>[2x]MKGQETRGFQSEVKQLLHLMIHSLYSNKEIFLRELISNASDAADKLRFRALSNPDLYEGDGELRVRVSFDKDKRTLTISDNGVGMTRDEVIDHLGTIAKSGTKSFLESLGSDQAKDSQLIGQFGVGFYS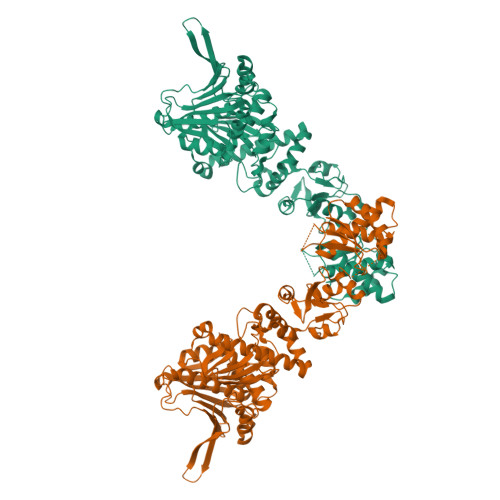AFIVADKVTVRTRAAGEKPENGVFWESAGEGEYTVADITKEDRGTEITLHLREGEDEFLDDWRVRSIISKYSDHIALPVEIEKREEKDGETVISWEKINKAQALWTRNKSEITDEEYKEFYKHIAHDFNDPLTWSHNRVEGKQEYTSLLYIPSQAPWDMWNRDHKHGLKLYVQRVFIMDDAEQFMPNYLRFVRGLIDSSDLPLNVSREILQDSTVTRNLRNALTKRVLQMLEKLAKDDAEKYQTFWQQFGLVLKEGPAEDFANQEAIAKLLRFASTHTDSSAQTVSLEDYVSRMKEGQEKIYYITADSYAAAKSSPHLELLRKKGIEVLLLSDRIDEWMMNYLTEFDGKPFQSVSKVDESLEKLADEVDESAKEAEKALTPFIDRVKALLGERVKDVRLTHRLTDTPAIVSTDADEMSTQMAKLFAAAGQKVPEVKYIFELNPDHVLVKRAADTEDEAKFSEWVELLLDQALLAERGTLEDPNLFIRRMNQLLVS> MAKTRPGVASKIKTGRKELDSYTIKGTNKVVRAGD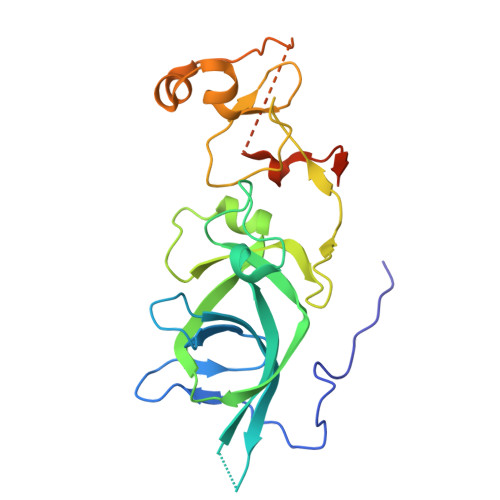CVLMRPSDAGKPPYVARVEKIEADARNNVKVHCRWYYRPEESLGGRRQFHGAKELFLSDHFDVQSAHTIEGKCIVHTFKNYTRLENVGAEDYYCRFEYKAATGAFTPDRVAVYCKCEMPYNPDDLMVQCEGCKDWYHPACVGMTIEEAKKLDHFVCAECSSDDDVAASQNGFTSSPADDVKVRLSLFSHLLYRCSITYL>NATTPTMQSTSLLTEHLGYPPISLVDDIINAVNEIMYKCTNAMEKYLMQRNIIGKKDFSDEIKIGT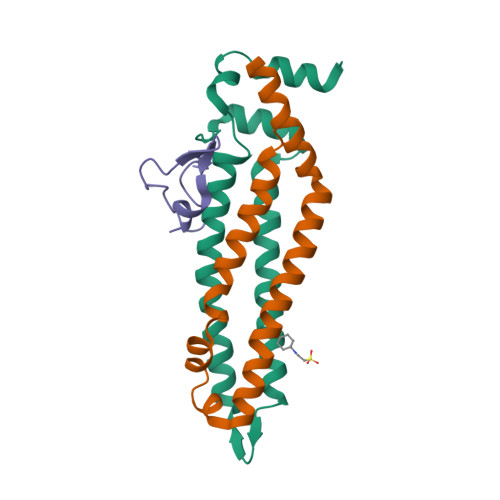AKLESLLENSVDKNFDKLELYVLRNILSIPSDLLEENRFRLLHHEKLVLTDSATR[2x];>MSVDRYSGMEGTEHIRFQRLVQVCNKALEESIRKLQSWEKIHECFPNYGQTREGIENLTVCQQQVIKLWSNLSRVEFDAIFHERSIEEKLNQLDDLINKARS[2x];>[2x]MDYMNLGVKSRKTGLTVNKTVQKDEYSMENLNDFFKDEQDS>MGSSHHHHHHSSGENLYFQGDLADRFAELERRYDARLGVYVPATGTTAAIEYRADERFAFCSTFKAPLVAAVLHQNPLTHLDKLITYTSDDIRSISPVAQQHVQTGMTIGQLCDAAIRYSDGTAANLLLADLGGPGGGTAAFTGYLRSLGDTVSRLDAEAPELNRDPPGDERDTTTPHAIALVLQQLVLGNALPPDKRALLTDWMARNTTGAKRIRAGFPADWKVIDKTGT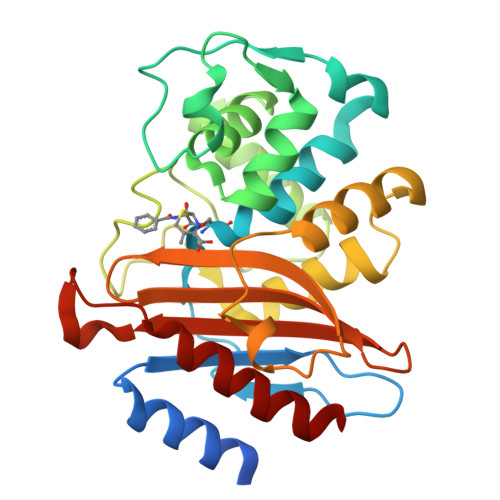GDYGRANDIAVVWSPTGVPYVVAVMSDRAGGGYDAEPREALLAEAATCVAGVLA[4x]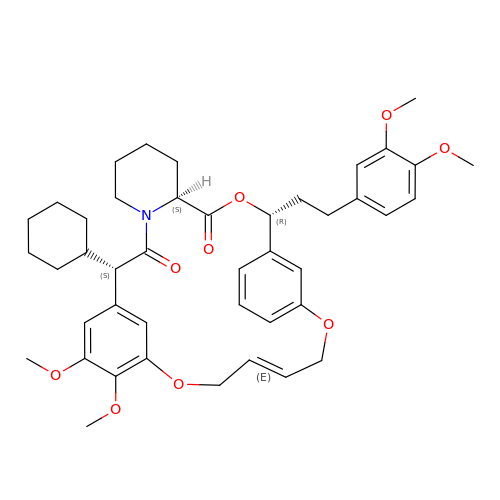2-cyclohexyl-12-[2-(3,4-dimethoxyphenyl)ethyl]-25,26-dimethoxy-11,18,23-trioxa-4-azatetracyclo[22.3.1.113,17.04,9]nonacosa-1(27),13(29),14,16,20,24(28),25-heptaene-3,10-dione | C43 H53 N O9 | NDUCBUBAJQQVOX-YBMMQTEXSA-N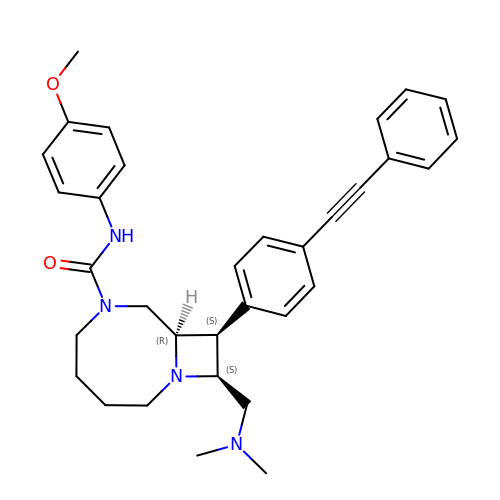(8R,9S,10S)-10-[(dimethylamino)methyl]-N-(4-methoxyphenyl)-9-[4-(2-phenylethynyl)phenyl]-1,6-diazabicyclo[6.2.0]decane-6-carboxamide | C33 H38 N4 O2 | VKRCTZCBMKVHCK-RTOKGZNSSA-N>[2x]ADQRRDFIDIESKFALRTPEDTAEDTCHLIPGVAESVATCHFNHSSKTFMVIHGWTVTGMYESWVPKLVAALYKREPDSNVIVVDWLSRAQEHYPVSAGYTKLVGQDVARFINWMEEEFNYPLDNVHLLGYSLGAHAAGIAGSLTNKKVNRITGLDPAGPNFEYAEAPSRLSPDDADFVDVLHTFTRGSPGRSIGIQKPVGHVDIYPNGGTFQPGCNIGEAIRVIAERGLGDVDQLVKCSHERSIHLFIDSLLNEENPSKAYRCSSKEAFEKGLCLSCRKNRCNNLGYEINKVRAKRSSKMYLKTRSQMPYKVFHYQVKIHFSGTESETHTNQAFEISLYGTVAESENIPFTLPEVSTNKTYSFLIYTEVDIGELLMLKLKWKSDSYFSWSDWWSSPGFAIQKIRVKAGETQKKVIFCSREKVSHLQKGKAPAVFVKCHDKSLNKKSG;>QTQQEEEEEDEDHGPDDYDEEDEDEVEEEE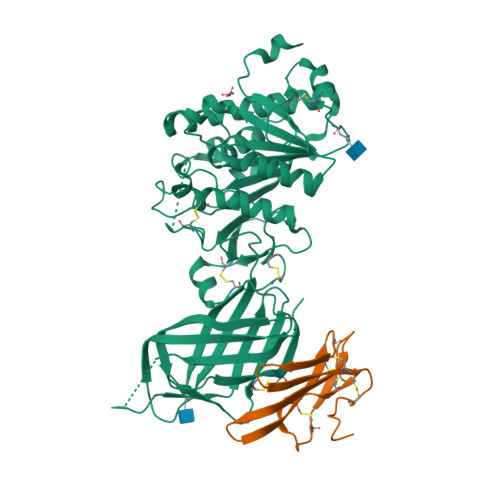TNRLPGGRSRVLLRCYTCKSLPRDERCDLTQDCSHGQTCTTLIAHGNTESGLLTTHSTWCTDSCQPITKTVEGTQVTMTCCQSSLCNVPPWQSSRVQDPTG[2x]5-nitrouracil | C4 H3 N3 O4 | 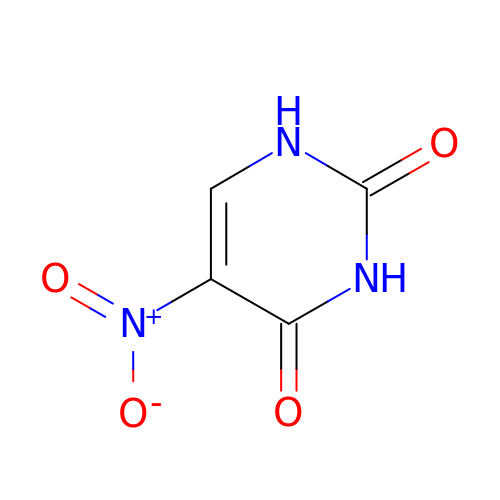TUARVSWVPPVUGS-UHFFFAOYSA-N>METGSFTVKTERRLQVLDVTGKVEEWLSTVGGVNGLLVVYVPHTTAAVAVNEAEPRLMEDIVEFIRELTKPGGPWKHNLVDVNAHAHLGNTIIGDSRVIPVVGGR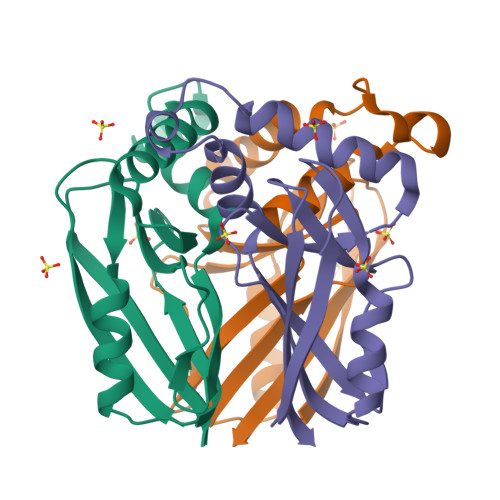LSLGTWQRILFVEMDGPRERTVNLLYLGE[2x]> SAFPVHAAFEKDFLVQLVVVDLNDSMDQVAEKVAYHCVNRRVAPREGVMRVRKHRSTELFPRDMTIAESGLNPTEVIDV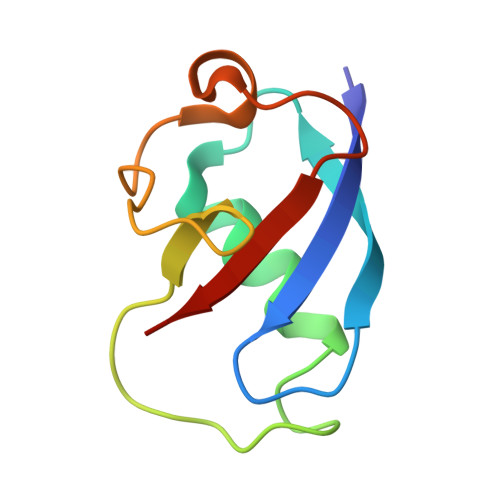VFEE>[4x]SMSVFAYE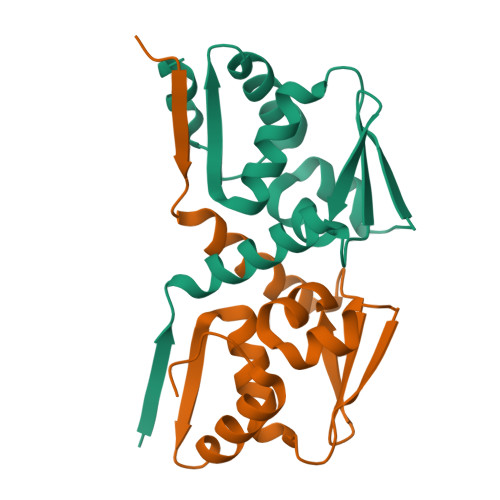SSVHSTNVLLSLNDQRKKDVLCDVTIFVEGQRFRAHRSVLAACSSYFHSRIVGQADGELNITLPEEVTVKGFEPLIQFAYTAKLILSKENVDEVCKCVEFLSVHNIEESCFQFLKF> MNAEINPLHAYFKLPNTVSLVAGS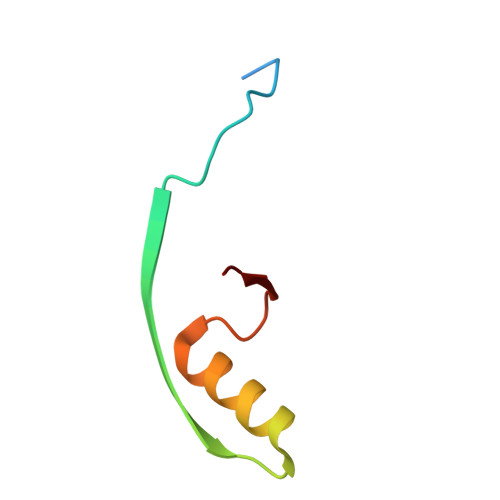SEGETPLNAFDGALLNAGIGNVNLIRIS> SYTRSEEIESLEQFHMATASSLIHKQMCSIVYTGPLKVQQMKNFIDSLVASLSAAVSNLVKILKDTAAIDLETRQKFGVLDVASKRWLVKPSAKNHAWGVVETHARKYHVALLEHDEFG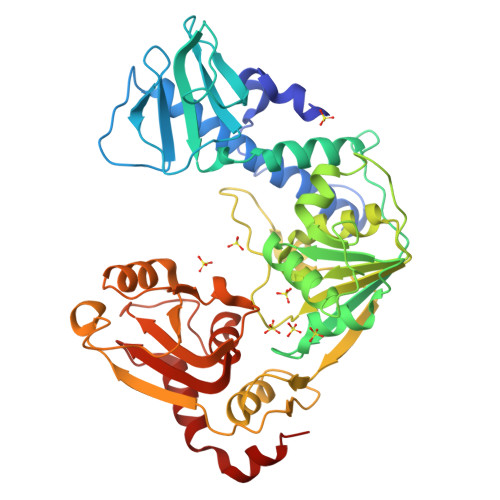IITCDNWRRVAVSSESVVYSDMAKLRTLRRLLKDGEPHVSSAKVVLVDGVPGCGKTKEILSRVNFEEDLILVPGRQAAEMIRRRANASGIIVATKDNVRTVDSFLMNYGKGARCQFKRLFIDEGLMLHTGCVNFLVEMSLCDIAYVYGDTQQIPYINRVTGFPYPAHFAKLEVDEVETRRTTLRCPADVTHFLNQRYEGHVMCTSSEKKSVSQEMVSGAASINPVSKPLKGKILTFTQSDKEALLSRGYADVHTVHEVQGETYADVSLVRLTPTPVSIIARDSPHVLVSLSRHTKSLKYYTVVMDPLVSIIRDLERVSSYLLDMYKV>[2x]MDVNLYGPGGPHTALKDIANKYSEKTGVKVNVNF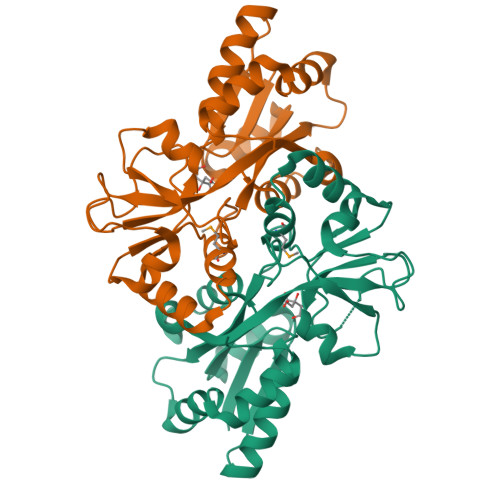GPQATWFEKAKKDADILFGASDQSALAIASDFGKDFNVSKIKPLYFREAIILTQKGNPLKIKGLKDLANKKVRIVVPEGAGKSNTSGTGVWEDMIGRTQDIKTIQNFRNNIVAFVPNSGSARKLFAQDQADAWITWIDWSKSNPDIGTAVAIEKDLVVYRTFNVIAKEGASKETQDFIAYLSSKEAKEIFKKYGWREHHHHHH> MTATPQGQIIHHRNFQSLYNNSWVCSLNVIKSRDGNNYSALEDITSDNQAFNNILEGIDIIECENLLKEMNVQKIPESSLFTNIKEALQAEVFNSTVEDNFESF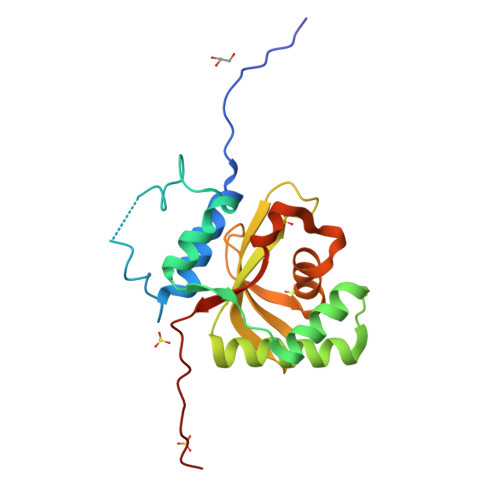ISYELQNHGPLMLIRPSLGSECLHAECIVGYDSEVKKVLIYDSMNTSPEWQSNIDVYDKLTLAFNDKYKNEDCSICGLYYDGVYEPKLEHHHHHH>MAAKLRKFLLRYYPPGIILQYERDGVMKQKPIDLLDLTPDVDVEVLLSQIIRQEPLISENRRPALRQLIHRLIDKMLEQQHHSFTLFKVLRAHILPLTNCAFNKSGDRFITGSYDRTCKVWNTFTGEEVFTLEGHKNVVYAIAFNNPYGDKIVTGSFDKTCKLWDAYTGQLYYTLKGHQTEIVCLSFNPQSTIIATGSMDNTAKLWDVETGQERATLAGHRAEIVSLGFNTGGDLIVTGSFDHDSRLWDVRTGQCV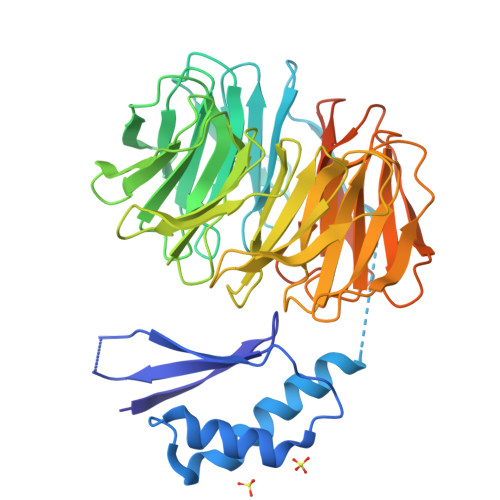HVLSGHRGEVSSTQFNYAGTLVVSGSIDCTSRLWDVRSGRCLSVKQGHTDEVLDVAFDAAGTKMVSASADGSARLYHTLTGVCQHTLVGHEGEISKVAFNPQGTRLITASSDKTCRLWDCDTGECLQVLEGHTDEIFSCAFNYEGDFIITGSKDNTCRIWKALTASSQPAGPGGAGGGLARPTTAFSYNDHHHHHH[2x]> DRVAQQANELIKRVAS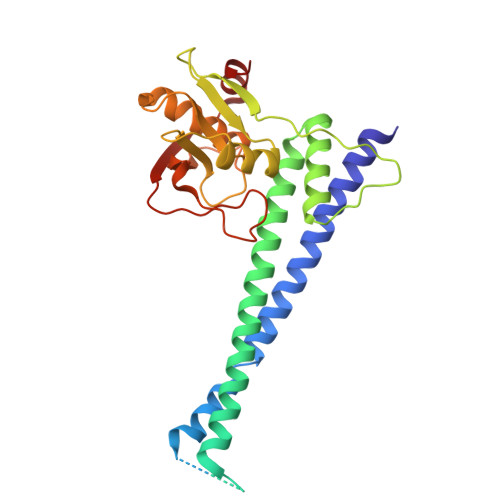ELEKNRKKLIKQEQELADTETAELVRQKGELLTTYVHQVPNDQSSVRLDNYYTGKELEIELDVALTPSQNAQRYFKKYQKLKEAVKHLTNLIEETKSTIVYLESVDTMLGQASLAEIDEIREELIETGYLKRRHREKIHKRQKPERYLATDGKTIILVGKNNLQNDELTFKMAKKGELWFHAKDIPGSHVVITDNLDPSDEVKTDAAELAAYFSKARHSNLVQVDMIEAKKLHKPTGGKPGFVTYRGQKTLRVTPTEDKIKSMKI> MTLELLQAQAQNCTACRLMEGRTRVVFGEGNPDAKLMIVGEGPGEEEDKTGRPFVGKAGQLLNRILEAAGIPREEVYITNIVKCRPPQNRAPLPDEAKI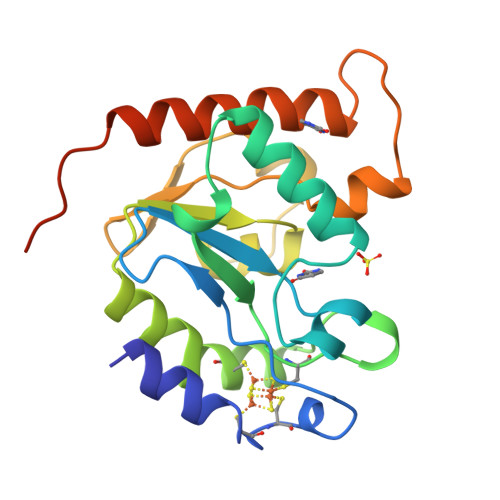CTDKWLLKQIELIAPQIIVPLGAVAAEFFLGEKVSITKVRGKWYEWHGIKVFPMFHPAYLLRNPSRAPGSPKHLTWLDIQEVKRALDALPPKERRPVKAVSQEPLF> MFCVQCEQTIRTPAGNGCSYAQGMCGKTAETSDLQDLLIAALQGLSAWAVKAREYGIINHDVDSFAPRAFFSTLTNVNFDSPRIVGYARE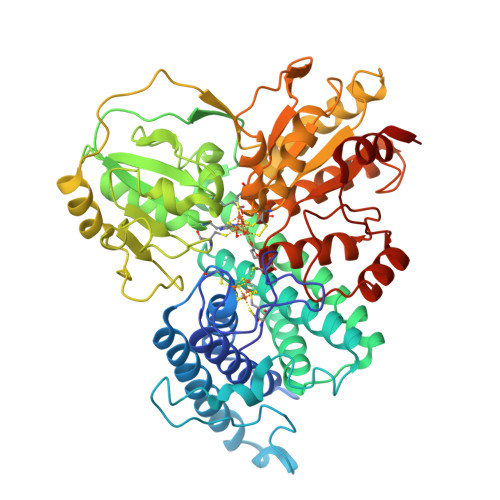AIALREALKAQCLAVDANARVDNPMADLQLVSDDLGELQRQAAEFTPNKDKAAIGENILGLRLLCLYGLKGAAAYMEHAHVLGQYDNDIYAQYHKIMAWLGTWPADMNALLECSMEIGQMNFKVMSILDAGETGKYGHPTPTQVNVKATAGKCILISGHDLKDLYNLLEQTEGTGVNVYTHGEMLPAHGYPELRKFKHLVGNYGSGWQNQQVEFARFPGPIVMTSNCIIDPTVGAYDDRIWTRSIVGWPGVRHLDGDDFSAVITQAQQMAGFPYSEIPHLITVGFGRQTLLGAADTLIDLVSREKLRHIFLLGGCDGARGERHYFTDFATSVPDDCLILTLACGKYRFNKLEFGDIEGLPRLVDAGQCNDAYSAIILAVTLAEKLGCGVNDLPLSLVLSWFEQKAIVILLTLLSLGVKNIVTGPTAPGFLTPDLLAVLNEKFGLRSITTVEEDMKQLLSALEHHHHHH> MLAKRIIACLNVKDGRVVKGTNFENLRDSGDPVELGKFYSEIGIDELVFLDITASVEKRKTMLELVEKVAEQIDIPFTVGGGIHDF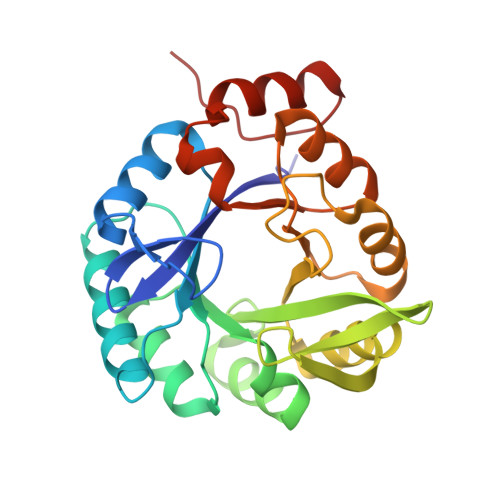ETASELILRGADKVSINTAAVENPSLITQIAQTFGSQAVVVAIDAKRVDGEFMVFTYSGKKNTGILLRDWVVEVEKRGAGEILLTSIDRDGTKSGYDTEMIRFVRPLTTLPIIASGGAGKMEHFLEAFLAGADAALAASVFHFREIDVRELKEYLKKHGVNVRLEGL>GSTSSVQRDDFHWEEYLKETGSISAPSECFRQSQIP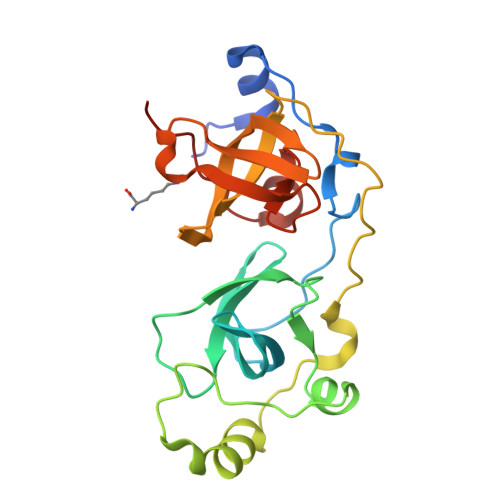PVNDFKVGMKLEARDPRNATSVCIATVIGITGARLRLRLDGSDNRNDFWRLVDSPDIQPVGTCEKEGDLLQPPLGYQMNTSSWPMFLLETLNGSEMASATLFKKEPPKPPLNNFKVGMKLEAIDKKNPYLICPATIGDVKGDEVHITFDGWSGAFDYWCKYDSRDIFPAGWCRLTGDVLQPPGTS[2x]>VPDLVY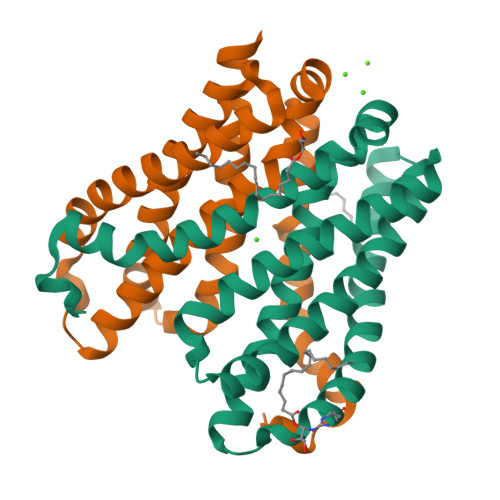SEAGPVALWLARVRWLVILILTGMVTSSILQGFESVLEAVTALAFYVPVLLGTGGNTGNQSATLIIRALATRDLDLRDWRRVFLKEMGVGLLLGLTLSFLLVGKVYWDGHPLLLPVVGVSLVLIVFFANLVGAMLPFLLRRLGVDPALVSNPLVATLSDVTGLLIYLSVARLLLEAV[2x]>[2x]APPSNLMQLPWRQGYSWQPNGAHSNTGSGYPYSSFDASYDWPRWGSATYSVVAAHAGTVR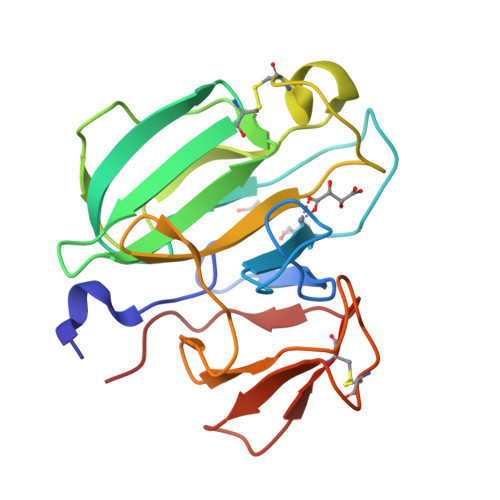VLSRCQVRVTHPSGWATNYYHMDQIQVSNGQQVSADTKLGVYAGNINTALCEGGSSTGPHLHFSLLYNGAFVSLQGASFGPYRINVGTSNYDNDCRRYYFYNQSAGTTHCAFRPLYNPGLAL> MATKSVLMLGSGFVTRPTLDVLTDSGIKVTVACRTLESAKKLSAGVQHSTPISLDVN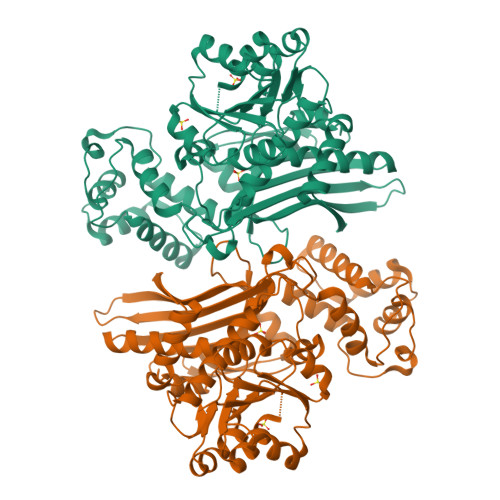DDAALDAEVAKHDLVISLIPYTFHATVIKSAIRQKKHVVTTSYVSPAMMELDQAAKDAGITVMNEIGLDPGIDHLYAIKTIEEVHAAGGKIKTFLSYCGGLPAPESSDNPLGYKFSWSSRGVLLALRNAASFYKDGKVTNVAGPELMATAKPYFIYPGFAFVAYPNRDSTPYKERYQIPEADNIVRGTLRYQGFPQFIKVLVDIGFLSDEEQPFLKEAIPWKEATQKIVKASSASEQDIVSTIVSNATFESTEEQKRIVAGLKWLGIFSDKKITPRGNALDTLCATLEEKMQFEEGERDLVMLQHKFEIENKDGSRETRTSSLCEYGAPIGSGGYSAMAKLVGVPCAVAVKFVLDGTISDRGVLAPMNSKINDPLMKELKEKYGIECKEKVVA>[2x]LFKSKAKAPKKVEKPKLKVEDGLFGTSGGIGFTKENELFVGRVAMIGFAASLLGEGITGKGILSQ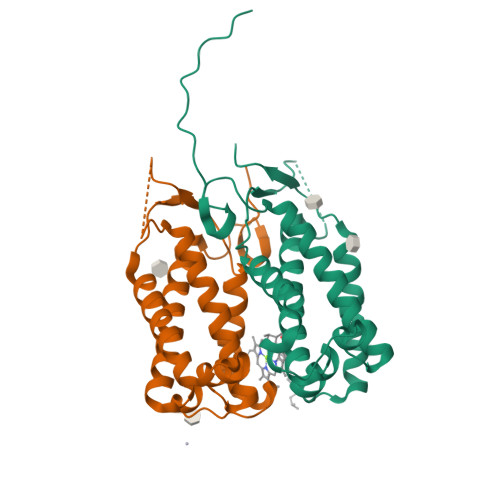LNLETGIPIYEAEPLLLFFILFTLLGAIGALGDRGRFVDEPTTGLEKAVIPPGKDVRSALGLKTKGPLFGFTKSNELFVGRLAQLGFAFSLIGEIITGKGALAQLNIETGVPINEIEPLVLLNVVFFFIAAINPGTGKFITDDEEED> GYGVEARGPTPEEAQREKDTRISKKMETMGIYFATPEWVALNGHRGPSPGQLKYWQN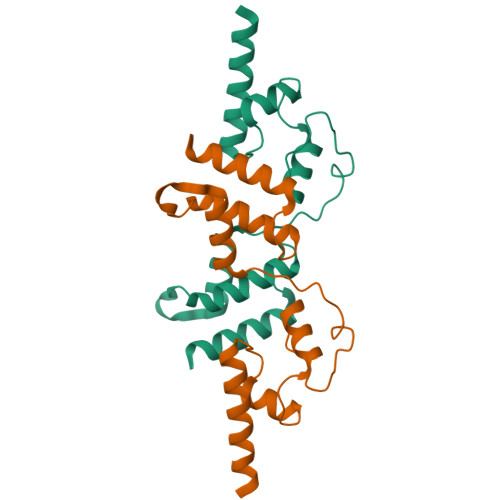TREIPDPNEDYLDYVHAEKSRLASEEQILRAATSIYGAPGQAEPPQAFIDEVAKVYEINHGRGPNQEQMKDLLLTAMEMKHR> MVELTEIKDDVVQLDEPQFSRNQAIVEEKASAT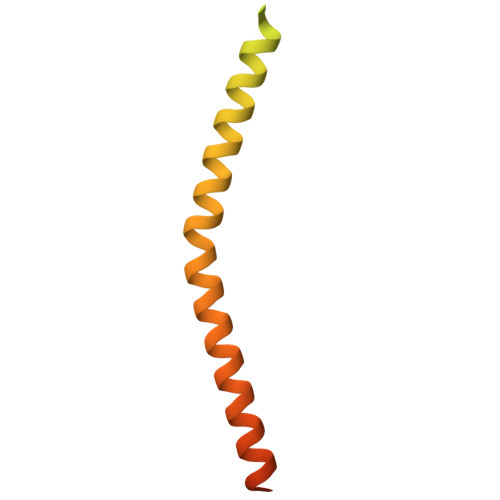NNDVVDDEDDSDSDFEDEFDENETLLDRIVALKDIVPPGKRQTISNFFGFTSSFVRNAFTKSGNLAWTLTTTALLLGVPLSLSILAEQQLIEMEKTFDLQSDANNILAQGEKDAAATAN> NTKYNKEFLLYLAGFVDSDGSIIAQIKPNQSVKFKHRLQLTFDVTQKTQRRWFLDKLVDEIGVGYVADSGSVSKYRLSEIKPLHNFLTQLQPFLKLKQKQANLVLKIIEQLPSAKESPDKFLEVCTWVDQIAALNDSKTRKTTSETVRAVLDS;> NTKYNKEFLLYLAGFVDGDGSIIAQIKPNQSGKFKHKLSLTFKVTQKTQRRWFLDKLVDEIGVGYVYDSGSVSNYYLSEIKPLHNFLTQLQPFLKLKQKQANLVLKIIEQLPSAKESPDKFLEVCTWVDQVAALNDSKTRKTTSETVRAVLDSL

I-CreI is a homodimeric member of LHEs family, which recognizes and cleaves a 22 bp pseudo-palindromic target (5′- CAAAACGTCGTGAGACAGTTTG -3′). Each I-CreI monomer binds its own DNA target region generating the catalytic centre at the dimer interface. This region contains two catalytic aspartic acids (D20, one per each monomer). The aspartic side chains participate in the cleavage of the DNA strands along the minor groove, resulting in the hydrolysis of specific phosphodiester bonds upon the coordination of three divalent metal ions.

To broaden our analysis, we also studied the I-CreI heterodimeric variant I-CreI_3115 (Y33G/Q38K/Q44K/R68Y/R70S/D75N/I77Y/I132V-G19S/Y33V/Q38R/S40Q/Q44D/R68A/R70S/D75K/I77R). This mutant was generated using the methodology previously described, and is able to recognize and cleave the human HBB (Haemoglobin beta subunit) gene (I-CreI_3115_target, Fig. 1c upper sequence) whose mutations cause sickle cell anaemia. To understand the molecular mechanism that inhibits cleavage when a G is at −4 position flanked by a pyrimidine at position −5, we solved the crystal structures of the cleavable and the corresponding non-cleavable variant targets in the presence of catalytic (Mg2+) and non-catalytic (Ca2+) cations. The MST measurements were then performed keeping constant the fluorescently labelled proteins and titrating the corresponding target DNAs in the presence of the non-catalytic cation Ca2+ (10 mM). This metal ion allows binding but hinders catalysis. To check this point, we analysed a superimposition of the crystal structures of both I-CreI variants bound to their target DNA sequences in the non-cleaved state.>DYADNDSILLKHGWCEMLKGGVIMDVKNVEQAKIAEKAGAIGVMILENIPSELRNTDGVARSVDPLKIEEIRKCISINVLAKVRIGHFVEAQILEELKVDMLDESEVLTMADEYNHINKHKFKTPFVCGCTNLGEALRRISEGASMIRTKGEAGTGNIIEAIKHIRTVNNEIKYLCSLDESEVYNFAKKLRAPIDLILLTRKLKRLPVVNFAAGGIATPADAAMCMQLGMDGVFVGSGIFESENPQKMASSIVMAVSNFNNPKILLNVSLGLGKAMHGNTAA[6x];>EITIGVLSLQGDFEPHINHFIKLQIPSLNIIQVRNVHDLGLCDGLVIPGGESTTVRRCCAYENDTLYNALVHFIHVLKKPIWGTCAGCILLSKNVENIKLYS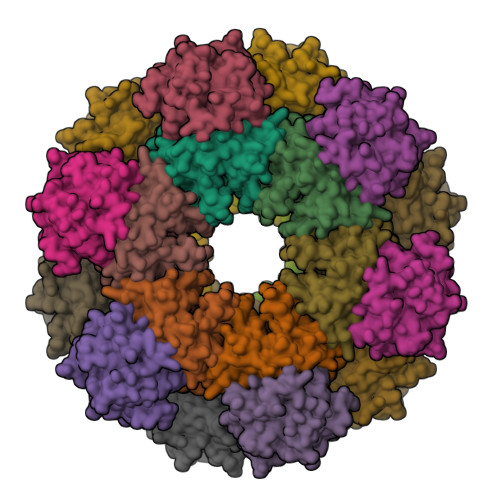NFGNKFSFGGLDITICRNFYGSQNDSFICSLNIISDSSAFKKDLTAACIRAPYIREILSDEVKVLATFSHESYGPNIIAAVEQNNCLGTVFNPELLPHTAFQQYFYEKVKNYKYS[6x]>[5x]SNAMIIRPEQHWFLRLFDWHGSVLSKIIFRLLLNVLMSIIAIISYQWYEQLGIHLTVAPFSLLGIAIAIFLGFRNSASYSRFVEARNLWGTVLIAERTLVRQLRNILPAEHDAHRRIVSYLVAFSWSLKHQLRKTDPTADLRRLLPEERVTEILASSMPTNRILLLAGNEIGQLREAGKLSDITYGLMDNKLDELAHVLGGCERLATTPVPFAYTLILQRTVYLFCTLLPFALVGDLHYMTPFVSVFISYTFLSWDSLAEELEDPFATAANDLPLNAMCNTIERNLLDMTGQHPLPE

Human bestrophin1 (hBest1) is a Ca2+-activated Cl− channel essential for Cl− transport in retinal pigment epithelium (RPE). Although the structure of hBest1 is still unsolved, two Best1 homolog structures, one from bacteria Klebsiella pneumoniae (KpBest) and the other from chicken (cBest1), have been previously reported. Overall, the channel is a pentameric assembly with a single ion-conducting pathway, which varies in diameter along its length and is constrained at two narrow points: a “neck” contributed by three residues (I62/I66/F70 in KpBest and I76/F80/F84 in hBest1/cBest1) on a transmembrane helix, and an “aperture” formed by a single residue (I180 in KpBest1, I205 in hBest1, and V205 in cBest1) on a cytosolic helix. Here, by electrophysiological and structural analyses, we show that the neck and aperture in hBest1 are both indispensable Ca2+-dependent gates, and their dysregulated opening by rationally designed or patient-derived mutations causes Ca2+-independent leak and elevates Ca2+-dependent channel activity.

Alanine substitution mutants for each of the 12 residues were generated in KpBest and hBest1 and subjected to crystallography and patch clamp, respectively. Moreover, the equivalent KpBest mutants (W16A, G18A, S19A, L259A, P262A, G264A, and D269A) all showed an overall similar structure to that of WT KpBest. The corresponding “Ca2+-binding” sites in WT KpBest are occupied by Zn2+, an essential component in the crystallization buffer. Interestingly, the KpBest P262A, G264A, and D269A mutants show no Zn2+ in the corresponding sites. In KpBest G264A, the methyl group of alanine, which is bulkier than glycine, may inhibit the binding of Zn2+. Moreover, KpBest L259A, P262A, G264A, and D269A all have relatively low resolution and slightly altered structures in this region, suggesting that the binding of Zn2+ stabilizes the channel structure.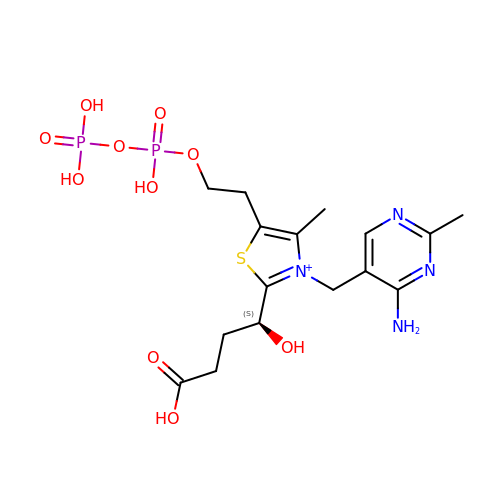(4S)-4-{3-[(4-amino-2-methylpyrimidin-5-yl)methyl]-5-(2-{[(S)-hydroxy(phosphonooxy)phosphoryl]oxy}ethyl)-4-methyl-1,3lambda~5~-thiazol-2-yl}-4-hydroxybutanoic acid | C16 H25 N4 O10 P2 S | RWCNVMPVYGBSHH-LBPRGKRZSA-N>MRGSHHHHHHGSMDRPFIFINSAMSADGKLSTKERKQVKISGKLNFERMDELRAHADAIMVGIGTVLADDPSLTVKSPERKAARKAAGKSENPVRVVVDSSARTPLNADIFKKGEGLRIIAVSNSAPEEKIRMLEEKALVIKTGAFRVDLTELAAKLKEMGINSLMVEGGATLNWGMLSAGLVDEVYTFVGNLIIGGKTAP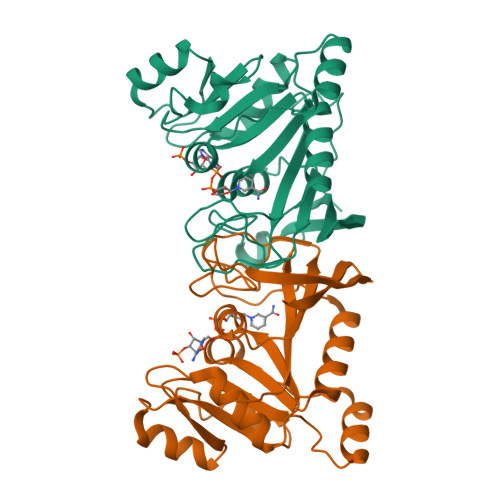TFTDGEGFTENELLGLELSSAEKIEDGILLKWKVKGKKN[6x]> MP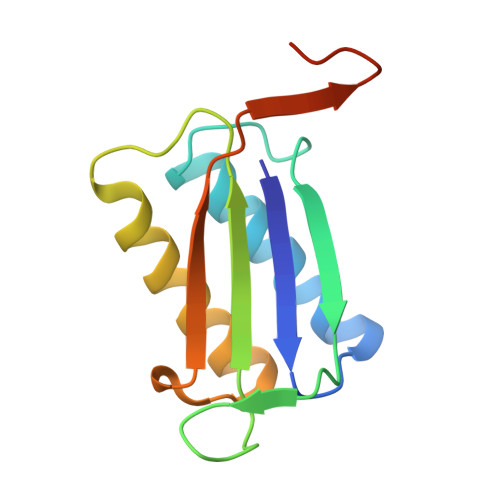VIQTFVSTPLDHEKRNMLTKVYRIVTDTILGKPAELVMMTFHDSTPMHFFGSTDPVACVRVEALGGYGPSEPEKVTKVVTDAISYVCGIVADRIFVLYFSPLHCGWNGTNLGSHHHHHH> GSHMTPKDDEFYQQWQLKYPKLILREASSVSEELHKEVQEAFLTLHKHGCLFRDLVRIQGKDLLTPVSRILIGNPGCTYKYLNTRLFTVPWPVKGSNIKHTEAEIAAACETFLKLNDYLQIETIQALEELAAKEKANEDAVPLCMSADFPRVGMGSSYNGQDEVDIKSRAAYNVTLLNFMDPQKMPYLKEEPYFGMGKMAVSWHHDENLVDRSAVAVYSYSCEGPEEESEDDSHLEGRDPDIWHVGFKISWDIETPGLAIPLHQGDCYFMLDDLNATHQHCVLAGSQPRFSSTHRVAECSTGTLDYILQRCQLALQNVCDDVDNDDVSLKSFEPAVLKQGEEIHNEVEFEWLRQFWFQGNRYRKCTDWWCQPMAQLEALWKKMEGVTNAVLHEVKREGLPVEQRNEILTAILASLTARQNLRREWHARCQSRIARTLPADQKPECRPYWEKDDASMPLPFDLTDIVSELRGQLLEA

FTO belongs to the family of Fe2+ and 2-oxoglutarate (2OG) dependent AlkB dioxygenases and contributes to non-syndromic human obesity. An m6A demethylase, FTO, was shown to regulate cellular levels of endogenous m6A residues, which strongly suggested that the m6A modification in mRNA is reversible and might be subject to dynamic regulation. Besides the internal m6A substrates in mRNA, FTO also oxidatively demethylates N3-methylthymine (dm3T) in single-stranded (ss) DNA and N3-methyluridine (m3U) in ssRNA in vitro, but has relatively lower activities compared to other AlkB family enzymes that catalyze a wide range of oxidative reactions. We performed a high-throughput fluorescence polarization (FP) assay to compare the differences in the displacement of m6A-containing ssDNA binding to FTO and ALKBH5, respectively, in the presence of compounds. This screening led directly to the discovery of meclofenamic acid (MA) that specifically inhibits FTO over ALKBH5.

In order to investigate the molecular recognition at atomic resolution, the structure of FTO in complex with the inhibitor MA was determined by crystallography in the presence of metal ion and N-Oxalylglycine (NOG), a chemical mimic of cofactor 2OG. MA was bound in the NTD region, and close to the interface of NTD and CTD. The binding site of MA is partially overlaid by dm3T- and rhein-binding sites. This explains the competitive property of MA binding to FTO over the m6A-containing nucleic acid. The metal ion is ligated by His231, Asp233 and His307, and bidentate NOG exists in an octahedral geometry. The following side chains come into contact with NOG: Asn205, Tyr295 and Arg316 through hydrogen bonding or salt bridge interactions. Hydrogen bonding occurs between the carboxyl group in MA and amides in Ser229 directly and Lys216 through a water molecule, respectively. One chlorine atom in MA directly contacts the complex guanidinium group in Arg96. In addition, the phenyl ring bearing carboxyl acid substituent forms hydrophobic interactions with the side chains of neighboring residues, Ile85, Leu90 and Pro93. Of note, the first loop in the FTO nucleotide recognition lid (NRL), β3i and β4i, which has been defined as the part of the NRL, provides hydrophobic interactions with inhibitor MA.>MELIRIAMKKDLENDNSLMNKWATVAGLKNPNPLYDFLNHDGKTFNEFSSIVNIVKSQYPDREYELMKDYCLNLDVKTKAARSALEYADANMFFEIEDVLIDSMISCSNMKSKEYGKVYKIHRELSNSVITEFEAVKRLGKLNIKTPEMNSFSRLLLLYHYLSTGNFSPMAQLIKQIDLSEISENMYIRNTYQTRVHVLMSNIKLNENSLEECREYSKKALESTNILRFQVFSYLTIGNSLLFSNYELAQENFLKG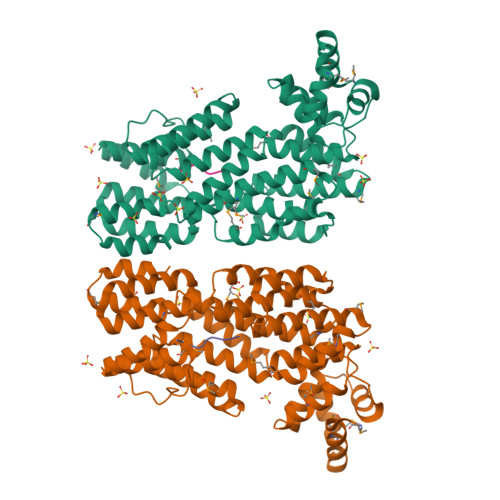LSISVQNENYNMIFQQALCFLNNVWRKENKWINFESDSIMDLQEQAHCFINFNENSKAKEVLDKLDLLVHNDNELAMHYYLKGRLEQNKACFYSSIEYFKKSNDKFLIRLPLLELQKMGENQKLLELLLL[2x];>[2x]GMPRGA Instead, SaPI derepression is facilitated by phage-encoded moonlighting proteins, which bind to the Stl repressor, activating the SaPI cycle. However, this assumption was incorrect, and we and others have recently demonstrated that the dUTP molecule blocks the Stl:Dut interaction, allowing us to propose a consensus model for Stl-Dut interaction where the apo form of the Duts provides the competent conformation for interacting with the Stl repressor. In this conformation motifs IV and VI provide the recognition and binding site for the Stl repressor, meanwhile the highly flexible motif V stabilizes the Stl-Dut complex once the repressor binds to the Dut.

Asp95 is responsible for chelating a divalent ion in the Dut threefold central channel, thus we produced this protein using two alternative protocols: the first of which included MgCl2 in the purification buffer, while the second did not, allowing us to evaluate the structural impact of this ion. We obtained crystals in the presence of a non-hydrolyzable dUTP analogue (dUPNPP) for both proteins, which present identical space group and cell dimensions to the previously reported crystals from wt Dut80α protein. However, the models built from the data obtained with the crystals produced with protein purified in the absence (Type I) or presence (Type II) of Mg ion showed small structural differences but with relevant mechanistic implications. The D95E mutation induces the reorientation of the new Glu side-chain in order to avoid the electrostatic repulsion between the carboxylate groups. In Type I crystals this is facilitated by a short movement consisting of the side-chain rotation of about 80° around Cβ atom that accommodates the Glu carboxylates deeper in the central channel, however in type II crystals the rotation is much smaller. This is because in Type II crystals a Mg ion occupies an almost identical position at the central part of the channel as was observed in the wt protein, while in Type I crystals the ion position is now occupied by a water molecule. In Dut80α D95E type I crystals where the Mg ion is absent, the conserved motif V that covers the active site was totally disordered, even though it was occupied by the nucleotide. In contrast, in Type II crystals, which retain the Mg ion, the motif V was visible over the active center with identical conformation to that observed in wild-type protein, but the density of the map was lower or even absent for some residues (Ser158, Gly164, Gly169 and Val170), supporting a weaker stabilization of this loop. Furthermore, Dut80α D95E Type I and II structures confirm the proposed allosteric effect between the threefold central channel and the active center, showing the fine correlation between Mg ion binding and motif V organization.

> MTNTLQVKLLSKNARMPERNHKTDAGYDIFSAETVVLEPQEKAVIKTDVAVSIPEGYVGLLTSRSGVSSKTHLVIETGKIDAGYHGNLGINIKNEHEDDKMQTIFLRNIDNEKIFEKERHLYKLGSYRIEKGERIAQLVIVPIWTPELKQVEEFESVSERGEKGFGSSGV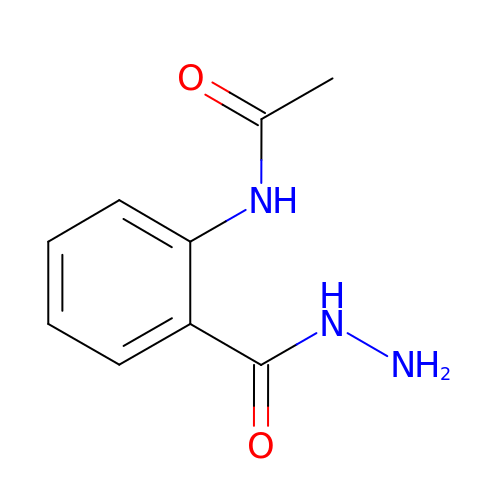~{N}-[2-(aminocarbamoyl)phenyl]ethanamide | C9 H11 N3 O2 | QECAIFFXHWSKAI-UHFFFAOYSA-N>GPMSRNDKEPFFVKFLKSS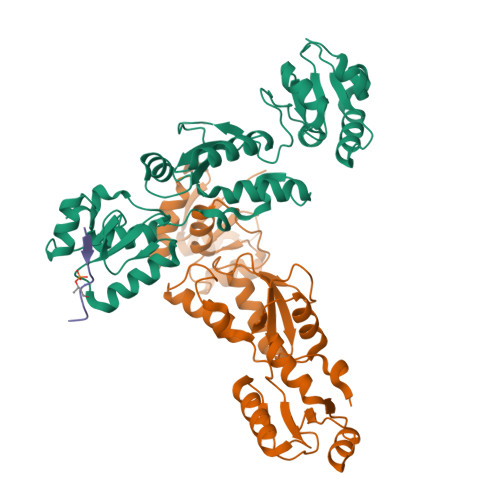DNSKCFFKALESIKEFQSEEYLQIITEEEALKIKENDRSLYICDPFSGVVFDHLKKLGCRIVGPQVVIFCMHHQRCVPRAEHPVYNMVMSDVTISCTSLEKEKREEVHKYVQMMGGRVYRDLNVSVTHLIAGEVGSKKYLVAANLKKPILLPSWIKTLWEKSQEKKITRYTDINMEDFKCPIFLGCIICVTGLCGLDRKEVQQLTVKHGGQYMGQLKMNECTHLIVQEPKGQKYECAKRWNVHCVTTQWFFDSIEKGFCQDESIYKTEPRPEA[2x];> EVEEIPETPCESQGE> MNHKVHHHHHHHHMSQWYELQQLDSKFLEQVHQLYDDSFPMEIRQYLAQWLEKQDWEHAANDVSFATIRFHDLLSQLDDQYSRFSLENNFLLQHNIRKSKRNLQDNFQEDPIQMSMIIYSCLKEERKILENAQRFNQAQ;> MNHKVHHHHHHHHMLETLINKIYTGPLGEELVQTLYLRIWAMEETPESLKILQMREDIRDQVLKMKTERWLRT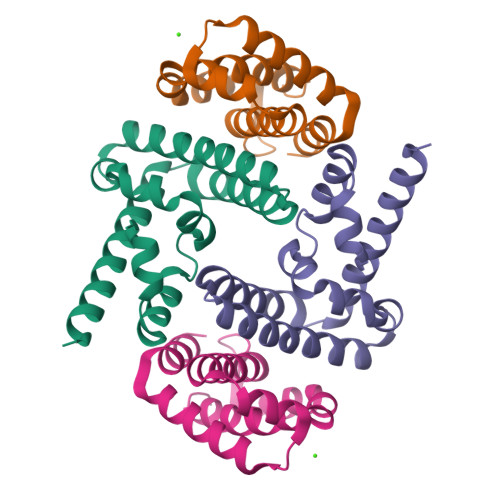LIRGEKTKLKDFQKRYEEVHPYLMKEKVEQVIMEEAWSLAAHIVQE> KANRQVSIT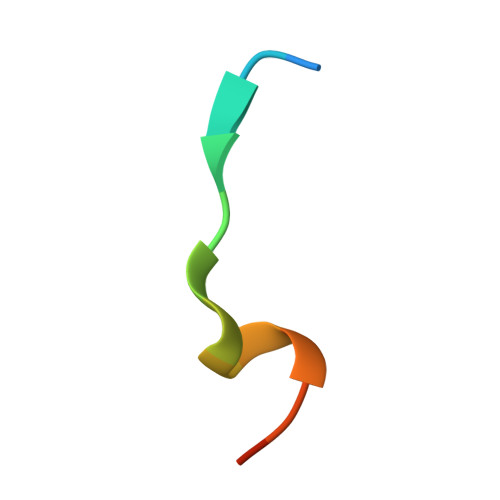GFFQRK>GKAFDDGVFTGIREINLSYNKE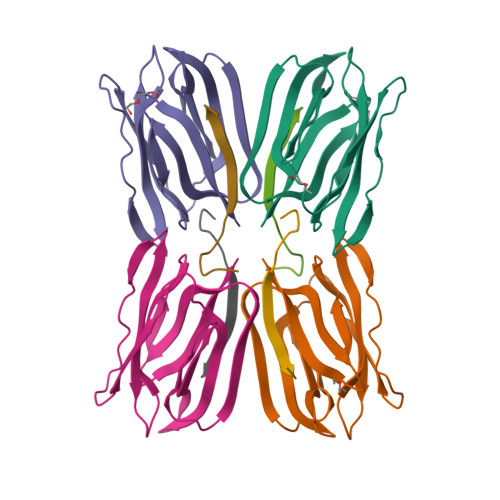TAIGDFQVVYDLNGSPYVGENHKSFITGFTPVKISLDFPSEYIMEVSGYTGKVSGYVVVRSLTFKTNKKTYGPYGVTSGTPFSLPIENGLIVGFKGSIGYWLDYFSMYLSL[8x];>NEQSGISQTVIVGPWGAQVST[8x]> SKRGNIPKP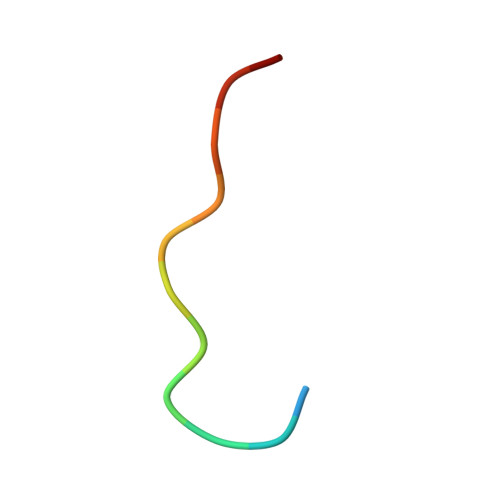LNLS4-chloranyl-~{N}-oxidanyl-1-benzothiophene-2-carboxamide 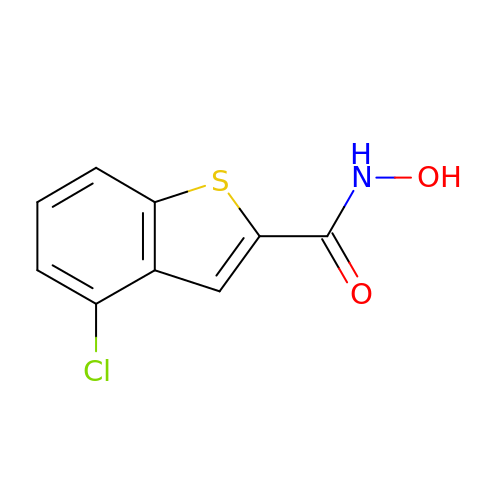| C9 H6 Cl N O2 S | IHGVZTXLHUWVIA-UHFFFAOYSA-N In the presence of NADH, acetoin is reduced to 2,3-BDO by the enzyme butanediol dehydrogenase (Bdh). SmBdh exhibits the typical single domain short-chain dehydrogenase/reductase (SDR) architecture. A monomer displays a dinucleotide-binding Rossmann fold that includes seven-stranded parallel β-sheet (β3–β2–β1–β4–β5–β6–β7) flanked by three α-helices (α2, α1, and α8) on one side and three α-helices (α3, α4, and α5) on another. There is an additional small lobe on top of a core structure, formed by two short helices, α6 and α7, creating a deep cleft in which the cofactor is bound, and where the active site is located.

In order to determine the importance of the Gln247 side chain for the catalysis, we developed two mutants of SmBdh: (1) Q247A where this side chain is removed, leaving alanine at position 247 and (2) the double mutant Q247A + V139Q, where the missing glutamine side chain would be reinstated at the position 139 that is present in KpBdh. The SmBdh Q247A and the Q247A + V139Q mutants crystallized in the same space group (P43212) as the WT SmBdh repeating its protein chains arrangement. As with the WT SmBdh, the primary difference between the two molecules in the asymmetric unit in the mutant structures was that molecule A was found in ‘closed’ conformation (that could be best described by ~ 10 Å distance between Cα-atoms of residues Ala93 and Trp192) and molecule B was found in ‘open’ conformation (the corresponding distance is ~ 15 Å). Upon examination of the electron density maps, we were able to locate NAD + cofactor molecule and a substrate in protein molecule A (‘closed’ conformation), whereas in molecule B (‘open’ conformation) the corresponding space is occupied by only adenine diphosphate (as in Q247A mutant) or remains unoccupied (as in Q247A + V139Q mutant) at all. In the Q247A mutant structure, a glycerol molecule was modeled at the substrate-binding pocket. Acetoin was present in the crystallization conditions, but our attempts to use additional acetoin for cryoprotection only led to crystal damage. Therefore, a 50/50 v/v mix of glycerol and ethylene glycol was used for cryoprotection. We postulate that the absence of the Gln247symm side chain led to an increase of the available space for the substrate and therefore the larger glycerol molecule could be bound. In comparison to the WT SmBdh, Q247A mutant showed a ~ 90% loss in activity as predicted by the structure, whereas the double mutant Q247A + V139Q showed ~ 300% improvement in activity in comparison to Q247A mutant. Although the double mutant did not completely restore the loss of Gln247 activity, significant function was regained by introducing the V139Q mutation in this protein. It can thus be inferred that Gln247 is extremely important for the activity of the protein, which cannot be fully restored by a complementary mutation, such as V139Q.

>MHHHHHHENLYFQGRFDNKVVVITGAGNGMGEAAARRFSAEGAIVVLADWAKEAVDKVAASLPKGRAMAVHIDVSDHVAVEKMMNEVAEKLGRIDVLLNNAGVHVAGSVLETSIDDWRRIAGVDIDGVVFCSKFALPHLLKTKGCIVNTASVSGLGGDWGAAYYCAAKGAVVNLTRAMALDHGGDGVRINSVCPSLVKTNMTNGWPQEIRDKFNERIALGRAAEPEEVAAVMAFLASDDASFINGANIPVDGGATASDGAPKIV[2x]>[4x]IISRNFPIIGVKEKTFEQLHKKCLEKKVLYVDPEFPPDE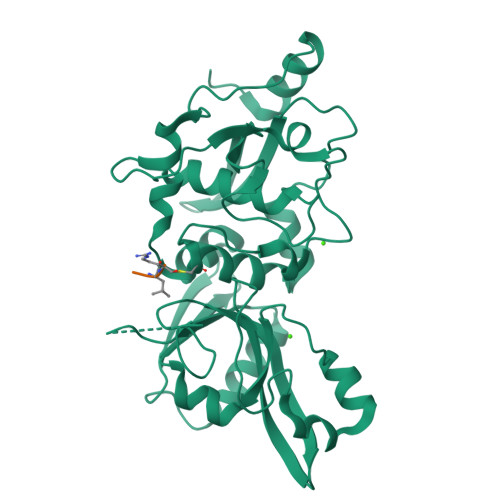TSLFYSQKFPIQFVWKRPPEICENPRFIIDGANRTDICQGELGDCWFLAAIACLTLNQHLLFRVIPHDQSFIENYAGIFHFQFWRYGEWVDVVIDDCLPTYNNQLVFTKSNHRNEFWSALLEKAYAKLHGSYEALKGGNTTEAMEDFTGGVAEFFEIRDAPSDMYKIMKKAIERGSLMGCSIDDGTNMTYGTSPSGLNMGELIARMVRNMDNSLLQDSDLDPRGSDERPTRTIIPVQYETRMACGLVRGHAYSVTGLDEVPFKGEKVKLVRLRNPWGQVEWNGSWSDRWKDWSFVDKDEKARLQHQVTEDGEFWMSYEDFIYHFTKLEICNLTADLEHHHHHH Here, we discovered a three-component monooxygenase system consisting of AibH1H2, AibG, and AibF for Aib hydroxylation in a Rhodococcus wratislaviensis strain possessing an oxygen-dependent Aib catabolic pathway not dependent on α,α-dialkylglycine decarboxylase. AibH1H2, a non-heme diiron enzyme, acts as the terminal oxygenase in the three-component monooxygenase system to produce α-methyl-d-serine (D-MeSer). All previously reported amino acid hydroxylases that form hydroxy groups on an aliphatic C–H bond belong to the Fe(II)/α-ketoglutarate-dependent dioxygenase (2OGDO) superfamily, but AibH1H2 belongs to the amidohydrolase superfamily (AHS). Thus, AibH1 and H2 are α′ and α subunits forming an α2α′2 heterotetrameric complex that act as the hydroxylase component in the Aib monooxygenase.

The crystal structure of AibH1H2 hydroxylase was determined to a resolution of 2.45 Å. AibH1H2 has a heterotetrameric structure of AibH1 and AibH2 subunits, and each subunit has the characteristic (β/α)8-barrel (TIM-barrel) fold present in all members of the AHS. The AibH1 and AibH2 subunits interact via 36 hydrogen bonds and numerous van der Waals interactions. The structures of AibH1 and AibH2 align well displaying a root-mean-square deviation of 1.75 Å for 294 residues, despite the overall amino acid identity of just 28%. In AibH2, the two Fe ions are coordinated by side-chains of three histidine and three carboxylate residues (Asp25H2, His27H2, His211H2, Glu265H2, Asp337H2, and His340H2), an ethylene glycol, and an oxygen atom. In the binuclear iron cluster containing oxygen bridges, the distances between Fe–O and Fe–Fe are 2.1/2.3 Å and 3.3 Å, respectively, and the Fe–O–Fe angle is 95°. AibH1 contains one Zn ion coordinated by side-chains of two histidine and three carboxylate residues (Asp24H1, His26H1, His201H1, Glu255H1, and Asp328H1). Thus, the AibH1H2 heterotetrameric complex contains two catalytic AibH2 subunits, each with a diiron center, and two AibH1 subunits, each containing a zinc ion. Although the amino acid sequence identity between AibH2 and Streptomyces platensis PtmU3 is only 25%, the residues needed to bind the Fe ions are highly conserved. The Glu313 of PtmU3 coordinates to an Fe ion, while the corresponding residue (Asp342) in AibH2 does not directly bind to, but indirectly interacts with, an Fe ion via a hydrogen bond network with water molecules replaced by ethylene glycol in the crystal structure.

> MRGSHHHHHHGSMVAPTSNPGVPDELDGVPAVVDCDVHAVLPSPHSLIPYLDEYWADQLVAQLAPTYEPNYHPRGSAIAQHSDASVDENGRAATTAENLVKDVFADGFTDFAVVNCLYGVQQIHQPRREMAHARALNHWIANEWLDKDDRLRASIVVPQGSPRAAAEEIDFWSGDKRFVQVLLLGQSELLYGREINWPIWEAAEAAGLPVTLHIGGVFRQAPTSVGWPASHLEWYVGQQSNIEAQLNSIISEGILQKFPKTKILLSELGFNWLPPFMWKFDKLWKSYRPDIPWVQESPLELIREHVRVTTSPSDGAEEAGRLDSIVDRLGSDRMLVYSSDYPHKHHSGPRDIENGTHSPELLDRIYRRNAFDLYNLVVPSPGKVG;> MTIIEHGSLGTLPAPSVTTGIVDADIHPVPQDGALEPYLDDRWKKHIREYGVRTTTGLQFISEYPQMYGGAMRADAWPESGYPGSDRELLRTQLLDKHNIQLGVLQCLAPGGQTLNPAGQALNQELAAALCRATNDWQLEHLVYPDPRMRAAIPVTFETPDYAVAEIERVGADPGVVAVLGTSKTLEPLGSRKYWPIYEASVAQNLPIQFHLSQGGGHANTGTGWTSYHTEYHTGHVQSFQSQLLSLVLSGTFDRFPTLKVMFVEGNVAHFAPLIQRMDYTWETLRGELPDLQRKPSEYIRDHIWASTQPIDEPEKPEHLAELLEEFCGDNVVFATDYPHFDFDDPETAFPRSFPVDLRDKILRGNGMRFFGVTNQAD>MKMMDANEIISFIQKSEKKTPVKVYIKGDLKEVTFPETVQAFVNKKSGVLFGEWSEIKTILDENSKYIVDYVVENDRRNSAIPMLDLKGIKARIEPGAIIRDHVEIGDNAVIMMNATINIGAVIGEGSMIDMNAVLGGRATVGKNCHVGAGAVLA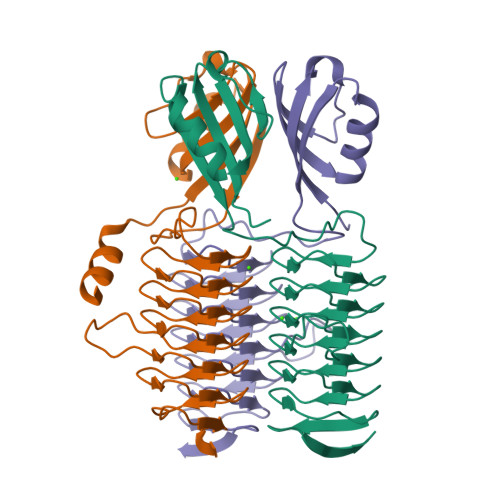GVIEPPSAKPVIVEDDVVIGANVVVLEGVTVGKGAVVAAGAVVTEDVPPYTVVAGTPARVIKEIDEKTKAKTEIKQELRQLNPEK[6x]>ARSTNTFNYATYHTLDEIYDFMDLLVAEHPQLVSKLQIGRSYEGRPIYVLKFSTGGSNRPAIWIDLGIHSREWITQATGVWFAKKFTEDYGQDPSFTAILDSMDIFLEIVTNPDGFAFTHSQNRLWRKTRSVTSSSLCVGVDANRNWDAGFGKAGASSSPCSE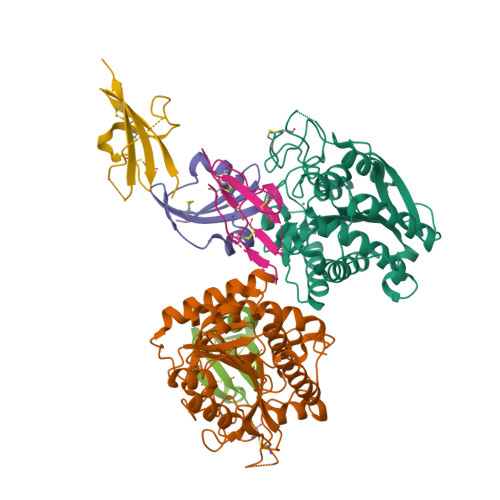TYHGKYANSEVEVKSIVDFVKDHGNFKAFLSIHSYSQLLLYPYGYTTQSIPDKTELNQVAKSAVAALKSLYGTSYKYGSIITTIYQASGGSIDWSYNQGIKYSFTFELRDTGRYGFLLPASQIIPTAQETWLGVLTIMEHTVNNLY[2x];>[4x]GSHTPDESFLCYQPDQVCAFICRGAAPLPSEGECNPHPTAPWAREGAVEWVPYSTGQCRTTCIPYVE> SGEKDVVFLIDGSEGVRSGFPLLKDFVQRVVESLDVGPDRVRVALVQYSDRTRPEFYLNSHMDQQGVISAIRRLTLLGGPTPNTGAALEFVLRNILTSSTGSRIAEGVPQLLIVLTAEPSGDDVRGPSVVLKQGGAVPIGIGIGNADISEMQTISFIPDFAVAIPTFRELGTIQQVISERVIQLNREELSSLKPILTPSTGAG

Collagen VI is a ubiquitously expressed extracellular matrix protein that forms a structurally unique network of beaded microfilaments. All collagen VI chains consist of a relatively short triple-helical region as well as of N- and C-terminal globular structures that are largely made up of VWA domains. Von Willebrand factor A (VWA) domains consist of about 200 amino acid residues and act as interaction modules in many intra- and extracellular proteins, e.g., in copines, integrins, von Willebrand factor, complement factors B and C2, matrilins, and collagens. The collagen VI α3N5 domain structure is the first solved structure of a collagen VWA domain and differs from other VWA domains in having an extended C-terminal region comprising residues N1206–G1224.

The murine collagen VI α3N5 domain was crystallized and its structure solved by molecular replacement at 1.2 Å resolution. The crystal asymmetric unit contains one molecule of collagen VI α3N5 comprising residues E1024–P1219. For the remaining five residues, S1220–G1224, poorer electron density precluded unambiguous model building. The structure has a central six-stranded hydrophobic β sheet flanked on either side by three amphipathic α helices. Like most of the collagen VI VWA domains, the α3N5 domain does not contain a conserved MIDAS motif. The C-terminal extension comprises a short α helix approximately at right angles with helix α6 followed by an extended region that cradles between the α4 and α5 helices of the N5 domain. Closer examination of the structure in this region shows that the extension is linked to the core domain by a salt bridge formed by residue R1207 from the C-terminal extension and E1024 from the core domain. Furthermore, residues L1210 and L1213 pack into a hydrophobic patch (patch 1; Figure 3, dark blue) formed by the residues P1130, L1132, V1158, and L1205 from the core domain, and a second hydrophobic patch (patch 2; Figure 3, light blue) is created by the side chains F1177, I1178, and P1179 from the core domain, which is buried by P1215 and I1216 from the C-terminal extension. The last two residues of the extension showing unique electron density, residues L1217 and P1219, interact with a hydrophobic ladder created by the long hydrophobic portions of the side chains of residues R1146, V1150, and K1153 of the α4 helix (green). As a result, the N and C termini are at opposite sides of the domain, which allows the formation of beads-on-a-string assemblies of multiple domains.> SQHMAFARDTEVYYENDTVPHMESIEEMYSKYA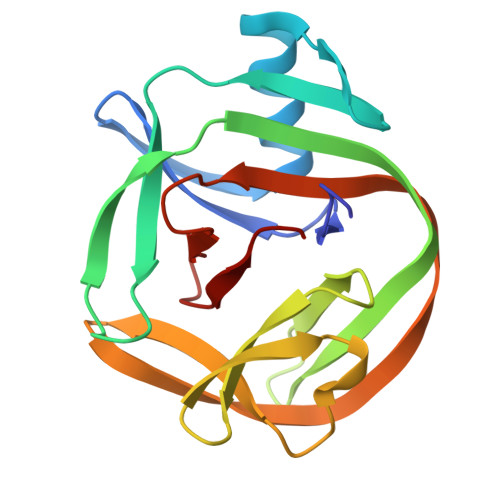SMNGELPFDNGYAVPLDNVFVYTLDIASGEIKKTRASYIYREKVEKLIEIKLSSGYSLKVTPSHPVLLFRDGLQWVPAAEVKPGDVVVGVRNGELEFHEVSSVRIIDYNNWVYDLVIPETHNFIAPNGLVLHNAQ> MACLASVALGSLHVEESLEMRFAAFKKKYGKVYKDAKEEAFRFRAFEENMEQAKIQAAANPYATFGVTPFSDMTREEFRARYRNGASYFAAAQKRLRKTVNVTTGRAPAAVDWREKGAVTPVKDQGQCGSAWAFSTIGNIEGQWQVAGNPLVSLSEQMLVSCDTIDFGCGGGLMDNAFNWIVNSNGGNVFTEASYPYVSGNGEQPQCQMNGHEIGAAITDHVDLPQDEDAIAAYLAENGPLAIAVDATSFMDYNGGILTSCTSEQLDHGVLLVGYNDASNPPYWIIKNSWSNMWGEDGYIRIEKGTNQCLMNQAVSSAVVGGPENLYFQ

Rhodesain is the lysosomal cathepsin L-like cysteine protease of Trypanosoma brucei rhodesiense, the causative agent of Human African Trypanosomiasis. The enzyme is essential for the proliferation and pathogenicity of the parasite as well as its ability to overcome the blood–brain barrier of the host. In the cell, cathepsins are expressed as inactive zymogens where the ∼215 amino acid papain-fold core protease domain is preceded by a ∼20 amino acid signal peptide required for translation of the protein into the endoplasmatic reticulum, and a ∼100 amino acid prodomain required for correct folding and lysosomal targeting of the protease. The prodomain interacts with the active site of the protease and keeps it in an autoinhibited state until it has been successfully trafficked to the acidic lysosome lumen.

To prevent autocleavage and to stabilize the proenzyme, we introduced a mutation into the active site of the protein, C150A. Here, we present the 2.8 Å crystal structure of the active site C150A mutant of the uncleaved T. brucei rhodesiense cysteine protease pro-rhodesain under acidic conditions. The proprotease structure contains two parts, the N-terminal prodomain (residues E38 to T123 according to uniprot numbering, ID.: Q95 PM0) and the C-terminal core protease domain (residues A126 to P342). The first 18 amino acids belonging to the prodomain, a short loop between the first two helices (residues 77/78) and residues G124/R125 at the C-terminus of the prodomain, are not resolved. The cleft between these domains harbors the active site triad residues C150 (mutated to alanine in our construct), H287 and N307. While the overall architecture of pro-rhodesain agrees with related proenzymes including human cathepsin L or C. papaya papain, pro-rhodesain displays a unique extended α-helix covering the entire cleft between the L- and R-lobes of the core protease domain. However, and so far unique to pro-rhodesain, a bulge forms around residues N103pro and G104pro, whose backbone amides are not involved in hydrogen bonds. Importantly, this bending of the α-helix enables the guanidino group of R100pro to interact with the side chain of Q144 in the core protease domain. In the pro-rhodesain structure, the S2’ and S1 sites are partially occupied by R100pro and S1’ by the side chain of Y101pro while a glycerol molecule sits in the center of the substrate-binding site. In contrast to the continuous α-helix observed for H3 in pro-rhodesain, the structures of all other available, nontrypanosomal pro-CathL proproteases display a mostly unstructured peptide in the C-terminal end of H3.> MSVTPKTLDMGAILADTSNRVVVCCGAGGVGKTTTAAALALRAAEYGRTVVVLTIDPAKRLAQALGINDLGNTPQRVPLAPEVPGELHAMMLDMRRTFDEMVMQYSGPERAQSILDNQFYQTVATSLAGTQEYMAMEKLGQLLSQDRWDLIVVDTPPSRNALDFLDAP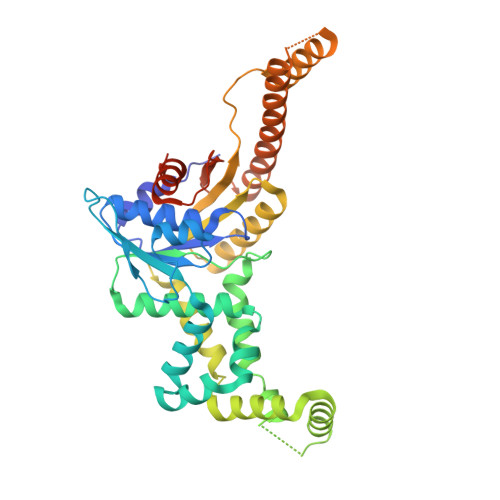KRLGSFMDSRLWRLLLAPGRGIGRLITGVMGLAMKALSTVLGSQMLADAAAFVQSLDATFGGFREKADRTYALLKRRGTQFVVVSAAEPDALREASFFVDRLSQESMPLAGLVFNRTHPMLCALPIERAIDAAETLDAETTDSDATSLAAAVLRIHAERGQTAKREIRLLSRFTGANPTVPVVGVPSLPFDVSDLEALRALADQLTTVGNDAGRAAGRLEHHHHHH>[3x]MSLNVKNDFSILIIEDDKEFADMLTQFLENLFPYAKIKIAYNPFDAGDLLHTVKPDVVMLDLMMVGMDGFSICHRIKSTPATANIIVIAMTGALTDDNVSRIVA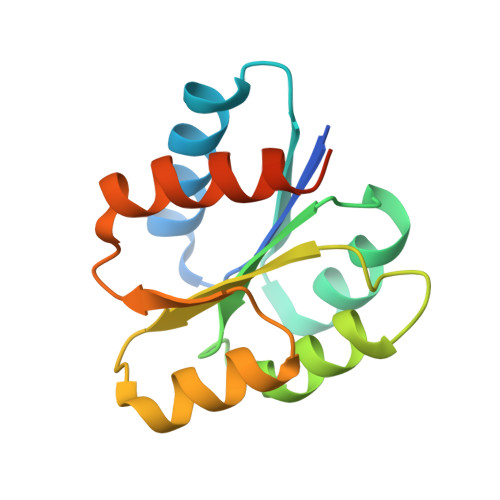LGAETCFGKPLNFTLLEKTIKQLVEQKKATSEGHHHHHH> SMGEIESYCNKELGPLPTKAPTLSKNV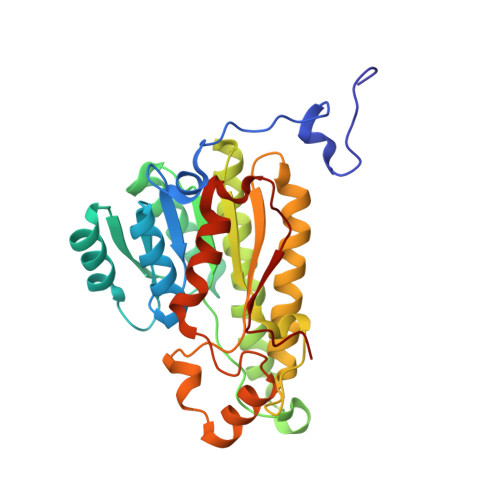LDLFSLKGKVASVTGSSGGIGWAVAEAYAQAGADVAIWYNSHPADEKAEHLQKTYGVRSKAYKCNISDPKSVEETISQQEKDFGTIDVFVANAGVPWTEGPEINVDNYDSWNKIINLDLNGVYYCAHTVGKIFKKNGKGSLVITSSMSGTIVNVPQLQAAYNAAKAACTHLTKSLAVEWAPFARVNCVSPGYIATEISDFVEKDMKAKWWQLTPLGREGLAQELVGAYLYLASNASTYTTGANLAVDGGYTCP>[2x]MKAYMFPGQGSQAKGMGRALFDAFPA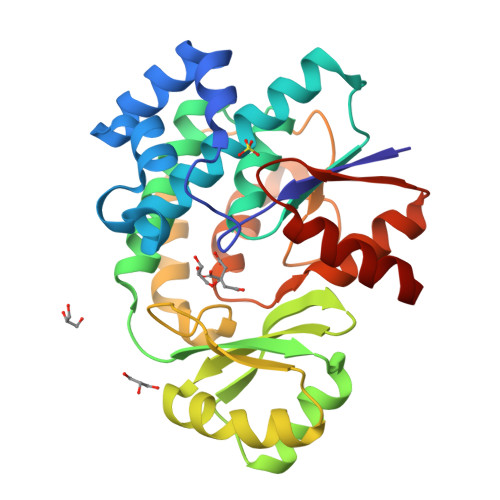LTARADGVLGYSIRALCQDDPDQRLSQTQFTQPALYVVNALSYLKRREEEAPPDFLAGHSLGEFSALFAAGVFDFETGLALVKKRGELMGDARGGGMAAVIGLDEERVRELLDQNGATAVDIANLNSPSQVVISGAKDEIARLQVPFEAAGAKKYTVLRVSAAFHSRFMRPAMVEFGRFLEGYDFAPPKIPVISNVTARPCKADGIRAALSEQIASPVRWCESIRYLMGRGVEEFVECGHGIVLTGLYAQIRRDA[[(2R,3S,4R,5R)-5-(6-aminopurin-9-yl)-4-oxidanyl-3-phosphonooxy-oxolan-2-yl]methoxy-oxidanyl-phosphoryl] [(3R)-2,2-dimethyl-3-oxidanyl-4-oxidanylidene-4-[[3-oxidanylidene-3-(propylamino)propyl]amino]butyl] 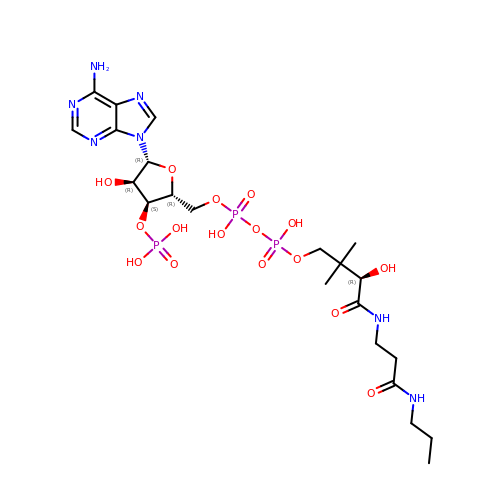hydrogen phosphate | C22 H38 N7 O16 P3 | JJSFSVFKDOGQNC-GORZOVPNSA-N>[2x]MTRAERKRQHINHALSIGQKRETGLDDITFVHVSLPDLALEQVDISTKIGELSSSSPIFINAMTGGGGKLTYEINKS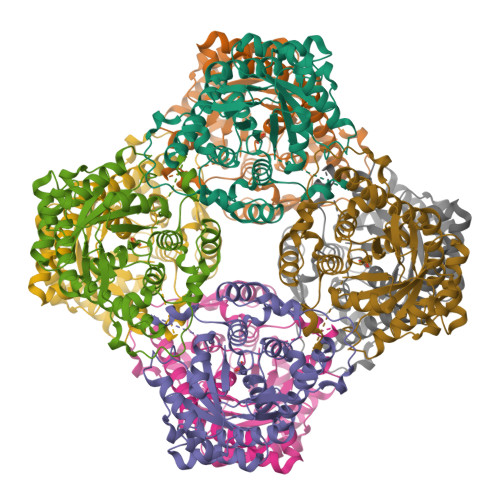LARAASQAGIPLAVGSQMSALKDPSERLSYEIVRKENPNGLIFANLGSEATAAQAKEAVEMIGANALQIHLNVIQEIVMPEGDRSFSGALKRIEQICSRVSVPVIVKEVGFGMSKASAGKLYEAGAAAVDIGGYGGTNFSKIENLRRQRQISFFNSWGISTAASLAEIRSEFPASTMIASGGLQDALDVAKAIALGASCTGMAGHFLKALTDSGEEGLLEEIQLILEELKLIMTVLGARTIADLQKAPLVIKGETHHWLTERGVNTSSYSVR1-methyl-1H-imidazole-5-carbaldehyde | C5 H6 N2 O | 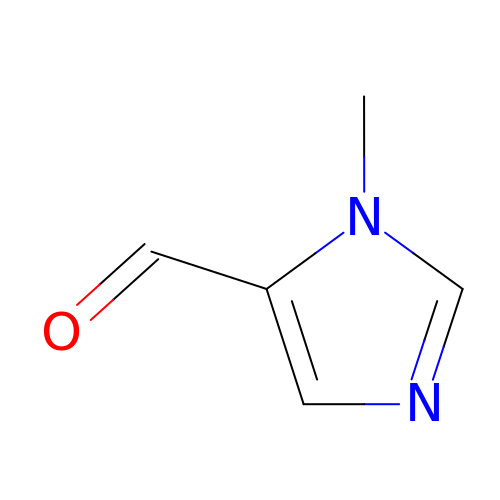BNYKZFOZWZMEJD-UHFFFAOYSA-N> MAHHHHHHMTELRPFYEESQSIYDVSDEFFSLFLDPTMAYTCAYFEREDMTLEEAQNAKFDLALDKLHLEPGMTLLDIGCGWGGGLQRAIENYDVNVIGITLSRNQFEYSKAKLAKIPTERSVQ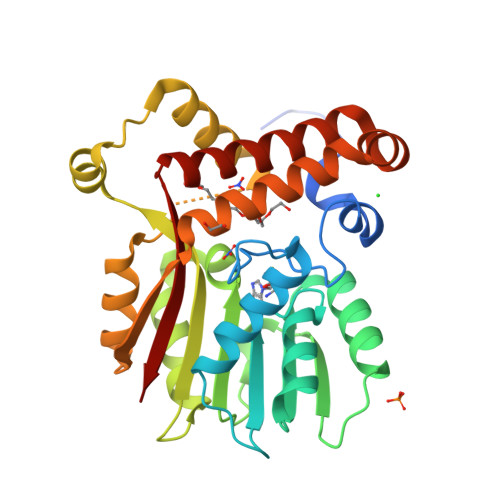VRLQGWDEFTDKVDRIVSIGAFEAFKMERYAAFFERSYDILPDDGRMLLHTILTYTQKQMHEMGVKVTMSDVRFMKFIGEEIFPGGQLPAQEDIFKFAQAADFSVEKVQLLQQHYARTLNIWAANLEANKDRAIALQSEEIYNKYMHYLTGCEHFFRKGISNVGQFTLTK> MAEVVNGKLHLRFAIAPMRPTPSQTIKEFEPIFKYLADQLGATYEIVSPESWAAISVAMTNGHVDVGWLGPWGYVLSNKKAGTEVLATVKYRGEPFYKALIVGRADLPIKKWPEDAKGLKLSLSDQGNTSGWLIPMAYFKSIGIDPASYFEYREGATFGQNESQIQHGLIDLGSDMDRGRNGMIEAGQIDPSKSKIVWESSKLPNAAISVPKDFDPALKARITEILTSLSEEKAQSLMGSGYNGFVKAKHSDYKVIEDAGRILGKLLEHHHHHH

P. stutzeri WM88 has PtxABC, HtxBCDE and PhnCDE ABC-transporters for the acquisition of phosphite, hypophosphite and organophosphonates, respectively. These transport systems rely on a high-affinity periplasmic binding protein (PBP) to impart ligand specificity. HtxB is a typical type-II PBP, with a binding pocket positioned in a deep groove between two domains separated by a hinge region. A comparison of the HtxB and PtxB structures showed that sequence differences within the binding pocket essentially eliminate an oxygen binding site in HtxB, providing specificity for a ligand with two oxygen atoms (hypophosphite), over one with three (phosphite).

To probe the role of the D206 in ligand binding we generated D206A and D206N mutants of HtxB. MST assays show that in the presence of 20 mM acetate the D206A mutant binds hypophosphite at both pH 7.4 and pH 5, but with a ca. 5000 × reduction in binding affinity compared to the WT protein in the same conditions. When we assayed D206A HtxB in acetate-free conditions at pH 7.4, no binding of hypophosphite could be detected up to 400 mM of ligand (data not shown). In the structure, the extra space generated by the alanine mutation allows for a single molecule of acetate to fulfill the role of D206 in the WT protein, forming two hydrogen bonds to R178, and a further hydrogen bond to the indole ring-nitrogen of W68. We cannot account for the origin of the acetate, but this explains why we only detect binding of hypophosphite to D206A HtxB via MST in acetate containing buffers. All of the atoms of the acetate molecule lie in plane of the guanidinium group of the arginine, forming a classic end-on salt bridge interaction. This differs from the direction of approach of the aspartate to the arginine in the WT complex, where the two oxygen atoms of the aspartate lie 1 Å below the plane of the guanidinium group, with the Cα-Cβ bond of D206 offset by approximately 75° from the same plane. The mode of binding of the hypophosphite and the degree of domain closure is the same as the WT protein (RMSD Cα: 0.19 Å), but the binding of the acetate slightly disrupts the local packing around the binding pocket, causing a change in rotamer conformation of M18. Clearly, the high concentration of hypophosphite in the crystallisation experiment along with the presence of acetate favours the formation of a closed, ligand-bound complex of D206A HtxB, that would not readily form in solution, given the weak binding affinity for ligand. However, the observation of acetate binding to facilitate the formation of the buried salt bridge in the closed complex of D206A HtxB, suggests that this intramolecular interaction is a prerequisite for capture of the ligand.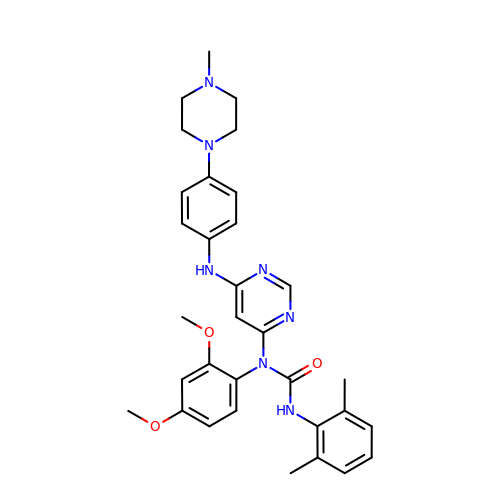1-(2,4-dimethoxyphenyl)-3-(2,6-dimethylphenyl)-1-[6-[[4-(4-methylpiperazin-1-yl)phenyl]amino]pyrimidin-4-yl]urea | C32 H37 N7 O3 | UYUHRKLITDJEHB-UHFFFAOYSA-N>[6x]MALDNLLRHLKISKEQITPVVLVVGDPGRVDKIKVVCDSYVDLAYNREYKSVECHYKGQKFLCVSHGVGSAGCAVCFEELCQNGAKVIIRAGSCGSLQPDLIKRGDICICNAAVREDRVSHLLIHGDFPAVGDFDVYDTLNKCAQELNVPVFNGISVSSDMYYPNKIIPSRLEDYSKANAAV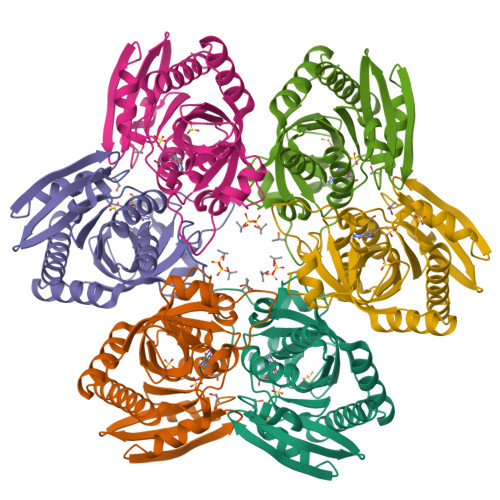VEMELATLMVIGTLRKVKTGGILIVDGCPFKWDEGDFDNNLVPHQLENMIKIALGACAKLATKYAKGEFEAYVEQKLISEEDLNSAVDHHHHHH>[4x]MMKPAKPLPKEMEEFVQSSGENGIVVFSLGSMISNMSEESANMIASALAQIPQKVLWRFDGKKPNTLGSNTRLYKWLPQNDLLGHPKTKAFITHGGTNGIYEAIYHG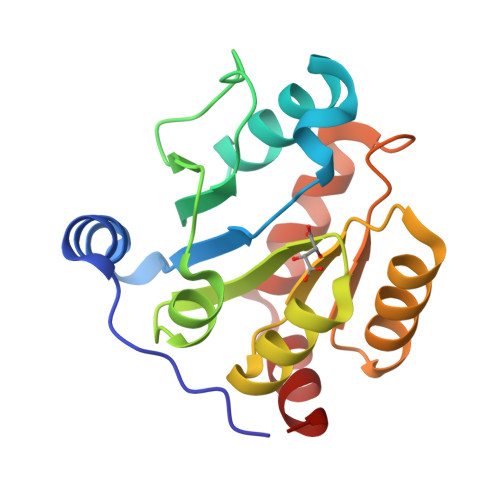IPMVGIPLFADQHDNIAHMKAKGAALSVDIRTMSSRDLLNALKSVINDPVYKENVMKSS Among the best characterized of the CYP152 family peroxygenases is the industrially relevant OleTJE (CYP152L1), first isolated from Jeotgalicoccus sp. ATCC 8456 in 2011 by Schirmer and co-workers. OleTJE acts primarily as a H2O2-dependent fatty acid decarboxylase to form terminal alkenes but also hydroxylates a proportion of these substrates to generate α- and β-hydroxylated fatty acids. Crystal structure data show that the active sites of OleTJE and P450 BSβ are very similar, with the carboxylate group of fatty acid substrates being coordinated by a conserved arginine residue (Arg245 in OleTJE, Arg242 in P450 BSβ, and Arg241 in P450 SPα). In this study, we explore further the structure and mechanism of OleTJE by mutating the key active site residues His85, Phe79, and Arg245 and by analyzing their effects on the catalytic properties of this biotechnologically important alkene-producing enzyme.

The importance of Phe79 in its interactions with His85 and in regulating active site structure and catalytic activity were explored by characterization of F79A, F79W, and F79Y variants. Crystals were obtained for both the H85Q and F79A mutant P450s in complex with arachidic acid substrate, as well as for the WT OleTJE in conditions containing formate. Structures for these mutant enzymes were determined to 1.44 Å (WT/formate), 1.80 Å (H85Q/arachidic acid) and 1.95 Å (F79A/arachidic acid). Arachidic acid substrate is bound similarly in both the H85Q and F79A mutants as was previously reported for the WT OleTJE. In contrast, for both OleTJE H85Q/F79A mutant structures, a sixth ligand water molecule is clearly visible. UV-visible substrate binding data for the H85Q/F79A mutants indicate much smaller HS shifts than observed for WT OleTJE, consistent with retention of the aqua-ligated LS state in the major fraction of the mutant P450s in the crystal structures. The F79A OleTJE mutant exhibited decreased activity compared with the WT and H85Q enzymes for all fatty acids tested. The alkenes are the major products with F79A OleTJE and all substrates, with the 3-hydroxylated fatty acid formed in excess over 2-hydroxyated fatty acids for the C10-C18 substrates. Mutations to OleTJE Phe79 also diminish substrate-dependent heme HS conversion and weaken affinity for shorter chain (C10:0-C16:0) fatty acid substrates. This translates into much lower product formation for the F79Y/W mutants from these substrates, although F79A OleTJE is less severely affected, with between 36 and 85% overall product formation compared with that of WT OleTJE for C10:0-C20:0 substrates. Crystal structure data for the H85Q and F79A mutants reveal only minor alterations to OleTJE active site structure, suggesting that quite subtle changes in the positions of active site amino acids, water molecule(s), and the substrate carboxylate region may be sufficient to trigger catalysis when H2O2 binds to initiate compound 0 formation.

>HHHHHHMATLKRDKGLDNTLKVLKQGYLYTTNQRNRLNTSVFQTKALGGKPFVVVTGKEGAEMFYNNDVVQREGMLPKRIVNTLAGKGAIHTVDGKKHVDRKALFMSLMTEGNLNYVRELTRTLWHANTQRMESMDEVNIYRESIVLLTKVGTRWAGVQAPPEDIERIATDMDIMIDSFRALGGAFKGYKASKEARRRVEDWLEEQIIETRKGNIHPPEGTALYEFAHWEDYLGNPMDSRTCAIDLMNTFRPLIAINRFVSFGLHAMNENPITREKIKSEPDYAYKFAQEVRRYYPFVPFLPGKAKVDIDFQGVTIPAGVGLALDVYGTTHDESLWDDPNEFRPERFETWDGSPFDLIPQGGGDYWTNHRCAGEWITVIIMEETMKYFAEKITYDVPEQDLEVDLNSIPGYVKSGFVIKNVREVVDRT[2x]>LDKLHVTSTRPQYVRIKNWGSGEILHDTLHHKATSDFTCKSKSCLGSIMNPKSLTRGPRDKPTPLEELLPHAIEFINQYYGSFKEAKIEEHLARLEAVTKEIETTGTYQLTLDELIFATKMAWRNAPRCIGRIQWSNLQVFDARNCSTAQEMFQHICRHILYATNNGNIRSAITVFPQRSDGKHDFRLWNSQLIRYAGYQMPDGTIRGDAATLEFTQLCIDLGWKPRYGRFDVLPLVLQADGQDPEVFEIPPDLVLEVTMEHPKYEWFQELGLKWYAL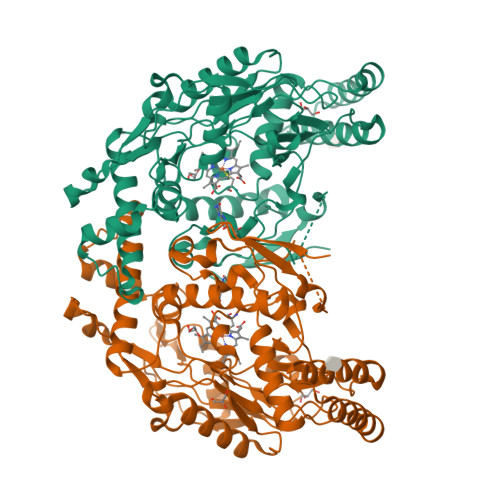PAVANMLLEVGGLEFPACPFNGWYMGTEIGVRDFCDTQRYNILEEVGRRMGLETHTLASLWKDRAVTEINVAVLHSFQKQNVTIMDHHTASESFMKHMQNEYRARGGCPADWIFLVPPVSGSITPVFHQEMLNYVLSPFYYYQIEPWKTHIWQNE[2x]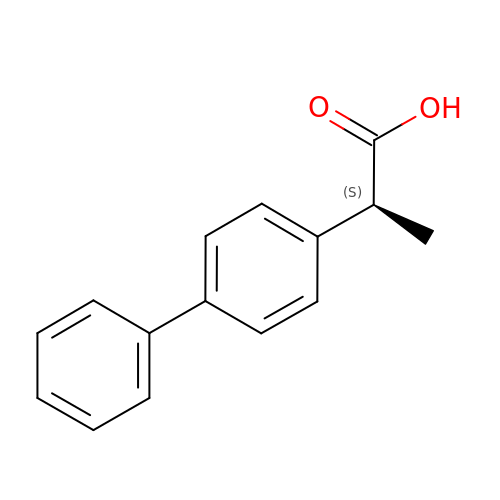2-(1,1'-BIPHENYL-4-YL)PROPANOIC ACID | C15 H14 O2 | JALUUBQFLPUJMY-NSHDSACASA-N>GIDPFTMTPSEDFVVTDRGGIVENSHRVHAAVVDAKGRLLYALGNPTRMTLARSAAKPAQA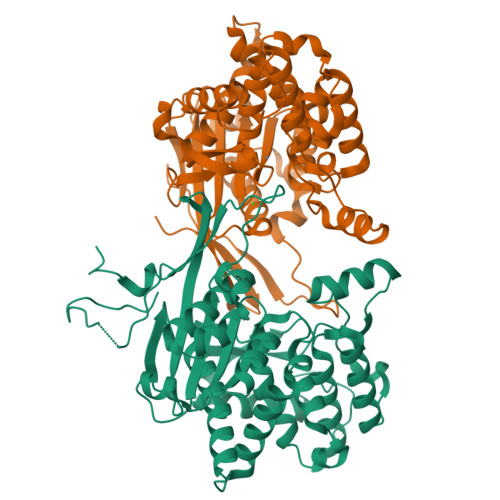LAILETEGVAGYGFDDADIALMCASHSSEDRHIARTRAMLSKIKAEEADLRCGGHPSLSEMVNRSWIKQDFIPTAVCSNCSGKHVGMLAGARAIGAGTDGYHLPDHPMQGRVKRTVAELCDLDAGDVEWGTDGCNLPTPAFPLDRLGRIYAKLASAADGSDAGEGQSTRCAALAHIFRAMARHPEMVAGEGRYCTMLMRAFDGALVGKLGADASYAIGVRASDATRQLGTDGALGISVKIEDGNLEMLYAVVTELLERLGIGSPDVRSQLASFHHPQRVNTMGVTTGGVSFPFKLRGSKSNVDDPRLAAVAR[2x]> PCYTATRSECKQKHKFVPGVWMAGEGMDVTTLRRSGSFPVNTQRFLRPDRTCTLCKNSLMRDATQRLPVAITHWRPHSSHCQRNVAAAKVHSTEGVAREAAANINNDWRVGLDVNPRPEANMRASVAGSHSKVANFAAEKTYQDQYNFNSDTVECRMYSFRLVQKPPLHLDFKKALRALPRNFNSSTEHAYHRLISSYGTHFITAVDLGGRISVLTALRTCQLTLNGLTADEVGDCLNVEAQVSIGAQASVSSEYKACEEK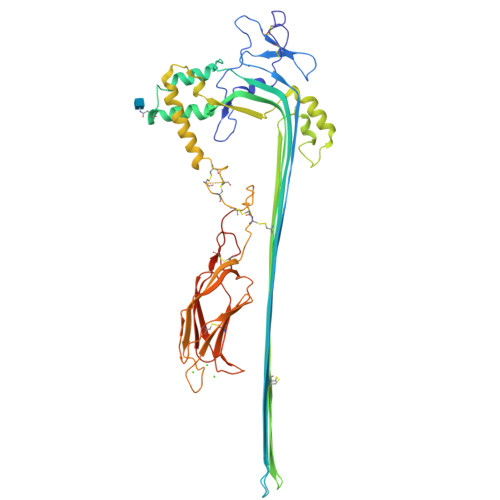KKQHKMATSFHQTYRERHVEVLGGPLDSTHDLLFGNQATPEQFSTWTASLPSNPGLVDYSLEPLHTLLEEQNPKREALRQAISHYIMSRARWQNCSRPCRSGQHKSSHDSCQCECQDSKVTNQDCCPRQRGLAHLVVSNFRAEHLWGDYTTATDAYLKVFFGGQEFRTGVVWNNNNPRWTDKMDFENVLLSTGGPLRVQVWDADYGWDDDLLGSCDRSPHSGFHEVTCELNHGRVKFSYHAKCLPHLTGGTCLEYAPQGLLGDPPGNRSGAVWHHHHHH>[2x]ERSSNNFNYGAYHSLEAIYHEMDNIAADFPDLARRV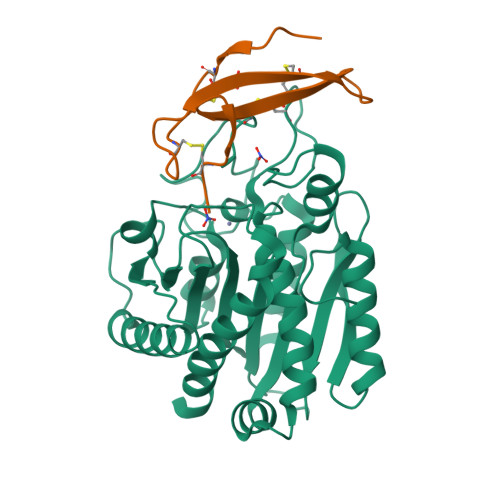KIGHSFENRPMYVLKFSTGKGVRRPAVWLNAGIHSREWISQATAIWTARKIVSDYQRDPAITSILEKMDIFLLPVANPDGYVYTQTQNRLWRKTRSRNPGSSCIGADPNRNWNASFAGKGASDNPCSEVYHGPHANSEVEVKSVVDFIQKHGNFKGFIDLHSYSQLLMYPYGYSVKKAPDAEELDKVARLAAKALASVSGTEYQVGPTCTTVYPASGSSIDWAYDNGIKFAFTFELRDTGTYGFLLPANQIIPTAEETWLGLKTIMEHVRDNLY;>[2x]FHVPDDRPCINPGRCPLVPDATCTFVCKAADNDFGYECQHVWTFEGQRVGCYA>[8x]GSHMKPASFMTSICDERGQELIYAGMPITEVFKEEMGIGGVLGLLWFQKRLPKYSCQFIEMCLMVTADHGPAVSGAHNTIICARAGKDLV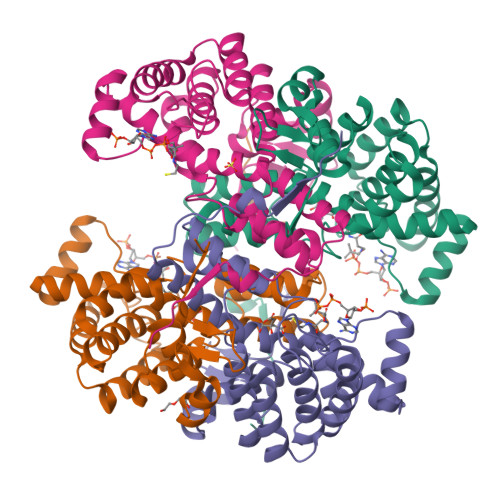SSLTSGLLTIGDRFGGALDAAAKMFSKAFDSGIIPMEFVNKMKKEGKLIMGIGHRVKSINNPDMRVQILKDYVRQHFPATPLLDYALEVEKITTSKKPNLILNVDGLIGVAFVDMLRNCGSFTREEADEYIDIGALNGIFVLGRSMGFIGHYLDQKRLKQGLYRHPWDDISYVLPEHMSM>MTAHRSVLLVVHTGRDEATETARRVEKVLGDNKIALRVLSAEAVDRGSLHLAPDDMRAMGVEIEVVDADQHAADGCELVLVLGGDGTFLRAAELARNASIPVLGVNLGRIGFLAEAEAEAIDAVLEHVVAQDYRVEDRLTLDVVVRQGGRI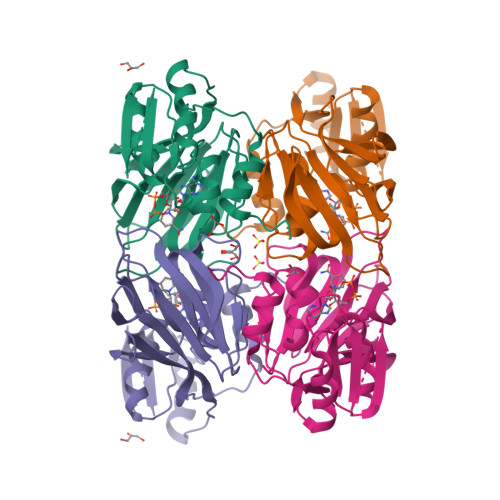VNRGWALNEVSLEKGPRLGVLGVVVEIDGRPVSAFGCDGVLVSTPTGSTAYAFSAGGPVLWPDLEAILVVPNNAHALFGRPMVTSPEATIAIEIEADGHDALVFCDGRREMLIPAGSRLEVTRCVTSVKWARLDSAPFTDRLVRKFRLPVTGWRGK[2x]MerTK, a TAM receptor, regulates macrophage efferocytosis and polarization, and its inhibition holds potential for tumor growth suppression and immune modulation. Additionally, MerTK plays a prominent role in regulating efferocytosis, the process by which macrophages engulf and clear apoptotic cells. MerTK is activated upon binding to its ligands, Protein S or growth arrest-specific 6 (GAS6), which recognize phosphatidylserine (PtdSer) exposed on the surface of apoptotic cell debris. In this study, we present a novel strategy for designing MerTK-selective inhibitors by modulating the conformational dynamics of its αC helix.

1 is a furo­[2,3-d]­pyrimidine-based pan-TAM inhibitor. In MerTK/1 complex structure, the crystal asymmetric unit contains two protein molecules, monomer A (chain A) and monomer B (chain B). 1 occupies the ATP binding site of each monomer and the binding of 1 induces the DFG out conformation of MerTK. The furo­[2,3-d]­pyrimidine core structure (Ring 4 and Ring 5) of 1 forms a hydrogen bond with M674 in the hinge region. The fluorobenzene (Ring 1) of 1 is positioned in the allosteric region, where it engages in extensive interactions with surroundings. Additionally, there is a C–F···C short contact between the fluorine atom of the benzene ring and the side chain carbon of L714 in the allosteric region. The 1-methylpyrazol-3-one (Ring-2) is situated between the DFG motif and the αC helix, where it forms a hydrogen bond with D741. Moreover, the carbonyl group at the amide linker forms a hydrogen bond with K619, thereby disrupting the conserved salt bridge between K619 in β strand and E637 in αC helix. In the structure of MerTK in complex with compound 1, the αC helix adopts two distinct conformations within the kinase dimer: monomer A assumes an’αC-in’ conformation, while monomer B adopts an’αC-out’ conformation.

>[2x]EELQNKLEDVVIDRNLLILGKILGEGEFGSVMEGNLKQEDGTSLKVAVKTMKLDNSSQREIEEFLSEAACMKDFSHPNVIRLLGVCIEMSSQGIPKPMVILPFMKYGDLHTYLLYSRLETGPKHIPLQTLLKFMVDIALGMEYLSNRNFLHRDLAARNCMLRDDMTVCVADFGLSKKIYSGDYYRQGRIAKMPVKWIAIESLADRVYTSKSDVWAFGVTMWEIATRGMTPYPGVQNHEMYDYLLHGHRLKQPEDCLDELYEIMYSCWRTDPLDRPTFSVLRLQLEKLLESLPDV>MANELTWHDVLAEEKQQPYFLNTLQTVASERQSGVTIYPPQKDVFNAFRFTELGDVKVVILGQDPYHGPGQAHGLAFSVRPGIAIPPSLLNMYKELENTIPGFTRPNHGYLESWARQGVLLLNTVLTVRAGQAHSHASLGWETFTDKVISLINQHREGVVFLLWGSHAQKKG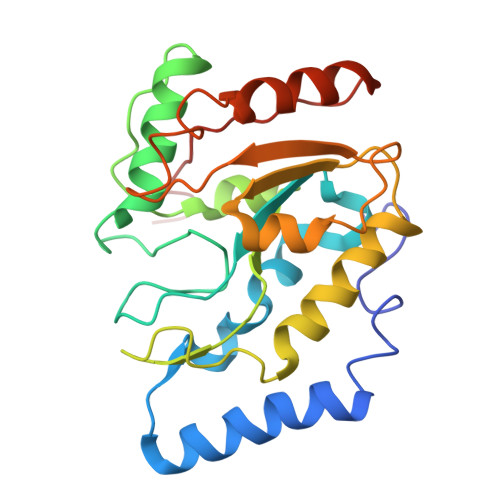AIIDKQRHHVLKAPHPSPLSAHRGFFGCNHFVLANQWLEQRGETPIDWMPVLPAESE[4x]> HMSGPSLQMSLHFSSMDREARVLRYREKKKARKFEKTIRYETRKAYAEARPRIKGRFAKRSDVQIEV;> MSPAKEQDRFLPIANVSRIMKRSLPANAKISKEAKETVQECVSEFISFVTGEASDKCQREKRKTINGDDLL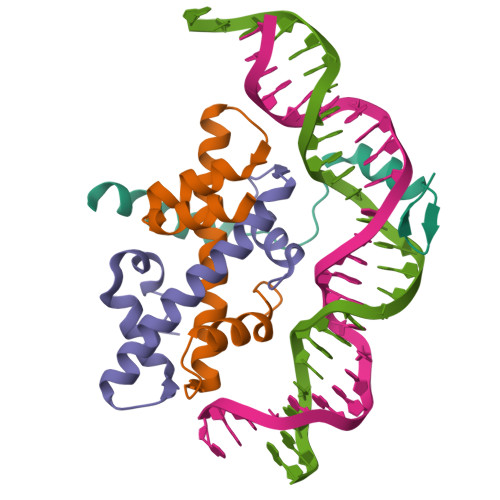WAMTTLGFEAYVGPLKSYLNRYRE;> HMQEAERASASDFKNHQLPLARIKKIMKADEDVRMISAEAPVLFAKACELFILELTIRSWLHAEENKRRTLQRNDVAAAIARTDVFDFLVDIVPREEAKEEPGS> MLSV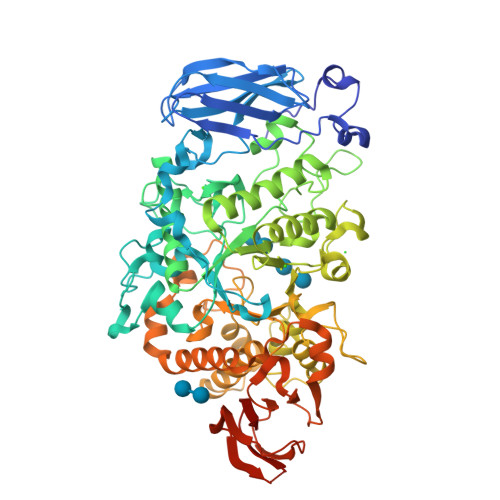QKEFHGTIDYGDVTVTGGISVFDAKFDELYVYDGDDLGAVYAPEETRFRLWAPTASEAFVVLYETEDGMPVKELPMKRDVQGTWTLTVAEDCGGLFYTYRVKVGEQWNEAVDPYAKAVGVNGTKTAILDLRSTNPEGWENDQKPPLASPTDAVIYELHVRDLSIHPQSGIREKGKFLGLTEEGTRGPNGIPTGLDHITGLGVTHVQLLPIYDYSQESVDESRLDEPHYNWGYDPQNYNVPEGSYSTDPHNPAARILELKRLIQKLHARGLRVIMDVVYNHVYDGYLIHFTKLVPGYYLRYKADRTFSDGTFCGNECASERPIMRKYIIESILHWVREYHIDGFRFDLMGMIDIETMNEIRRRLDEIDPTILTIGEGWMMETVLPKELRANQDNAEKLPGIGMFNDGMRDAVKGDIFIFDRKGFISGGDGFEDGVKRGVAGGINYGGQLRQFAVEPVQSVNYVECHANHTLWDKIELSTPGASDEERRAMHRLASAIVLTSQGIPFLHAGQEFMRTKGGVENSYKSPIEVNWLDWERCAAHQDDVSYMRSLIALRKAHPAFRLKTADEIRAHLRFEAAPPHTVAFTLRDHAGGDPDRHLYVLYNANPGALSLELPALGPWEVRFGGEHVLALEAGASGEAAAAAPAAAGGPPAGGARLEVRGVGVVVLAVPR>[4x]GSHMAT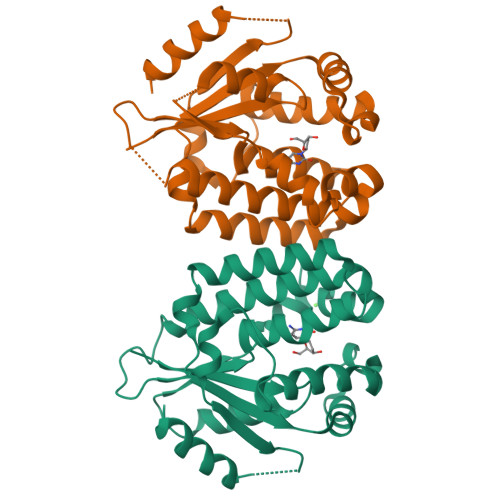PPKRSCPSFSASSEGTRIKKISIEGNIAAGKSTFVNILKQLCEDWEVVPEPVARWCNVQSTNVLQMMYEKPERWSFTFQTYACLSRIRAQLASLNGKLKDAEKPVLFFERSVYSDRYIFASNLYESECMNETEWTIYQDWHDWMNNQFGQSLELDGIIYLQATPETCLHRIYLRGRNEEQGIPLEYLEKLHYKHESWLLHRTLKTNFDYLQEVPILTLDVNEDFKDKYESLVEKVKEFLSTL>[2x]MENNGIDGVVLYEDADHKFIWLGSESKQRKGAVQTMQYLIVDRGRGVLL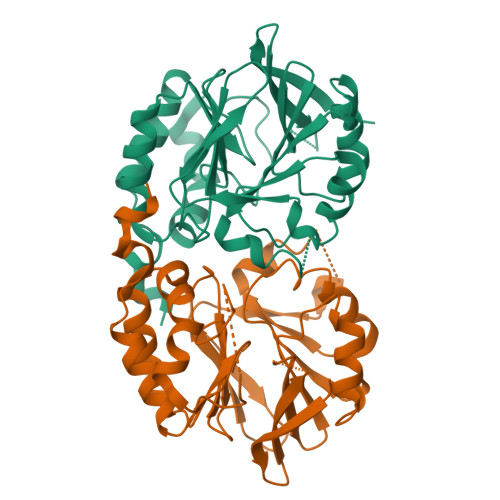DPGGVHLFSRVVTAISRFISVDKIDTIFFSHQDPDVSSGIALWLGITKAKIYISSLWVRFMPHFGIVDISRMVPIPDKGMSISLPSGSNMKCIPSHFMHSPGQFGLYDERSRILFSGDIGAAVFDDDNETTFVEDFEKHLPLIEGFHVRYMASNKIVSKWVEYVRRLNPLMIAPQHGAIYKDEQVNNFLNWLSGLKCGTDYIENLF>MRGSHHHHHHGMASH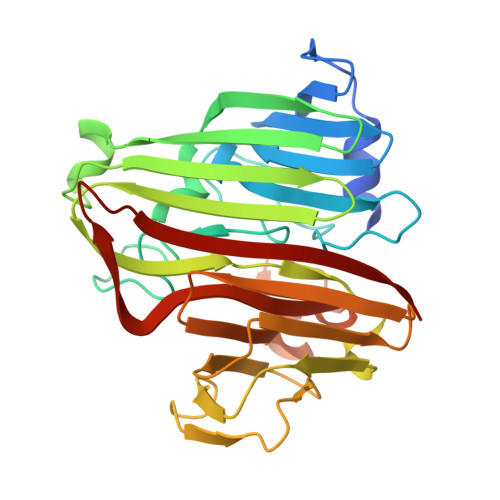MINKIFALPVIEQLTPVLSRRQLDDLDLIVVDHPQVKASFALQGAHLLSWKPVGEEEVLWLSNNTPFKTGVALRGGVPICWPWFGPAAQQGLPSHGFARNLPWALKAHNEDDNGVMLTFELQSSEATRKYWPHDFTLLARFKVGKTCEIELEAHGEFATTSALHSYFNVGDIANVKVSGLGDRFIDKVNDAKEGVLTDGIQTFPDRTDRVYLNPEACSVIHDATLNRTIDVVHHHHLNVVGWNPGPALSVSMGDMPDDGYKTFVCVETVYATAPQQATEEKPSRLAQTICVAKR[4x]> APLAHTHQDFQPVLHLVALNTPLSGGMRGIRGADFQCFQQARAVGLSGTFRAFLSSRLQDLYSIVRRADRGSVPIVNLKDEVLSPSWDSLFSGSQGQLQPGARIFSFDGRDVLRHPAWPQKSVWHGSDPSGRRLMESYCETWRTETTGATG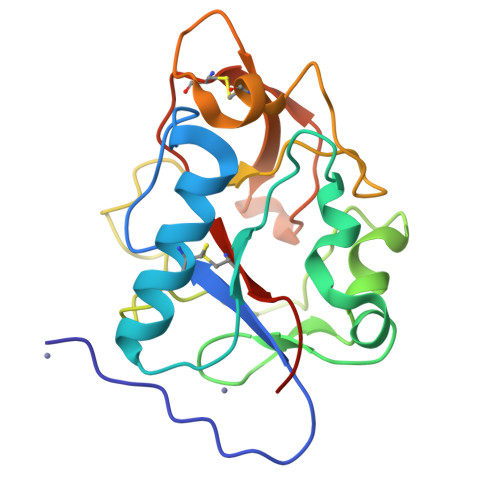QASSLLSGRLLEQKAASCHNSYIVLCIENSFMTSFSK4,4'-(5-{[(1H-imidazol-4-yl)methyl]amino}-1H-pyrazole-3,4-diyl)diphenol 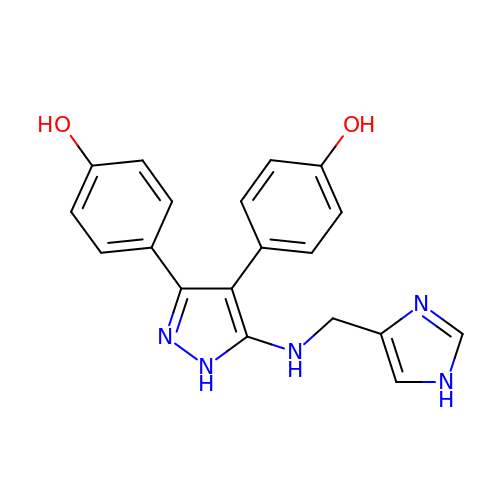| C19 H17 N5 O2 | QNVXUJBXEJSMQO-UHFFFAOYSA-N>MGSLVCVGTGLQLAGQISVLSRSYIEHADIVFSLLPDGFSQRWLTKLNPNVINLQQFFAQNGEVKNRRDTYEQMVNAILDAVRAGKKTVCALYGHPGVFACVSHMAITRAKAEGFSAKMEPGISAEACLWADLGIDPGNSGHQSFEASQFMFFNHVPDPTTHLLLWQIAIAGEHTLTQFHTSSDRLQILVEQLNQWYPLDHEVVIYEAANLPIQAPRIERLPLANLPQAHLMPISTLLIPPAKKLEYNYAILAKLGIGPEDLG[2x];>[2x]MSGLSDFFTQLGQDAQLMEDYKQNPEAVMRAHGLTDEQINAVMTGDMEKLKTLSGDS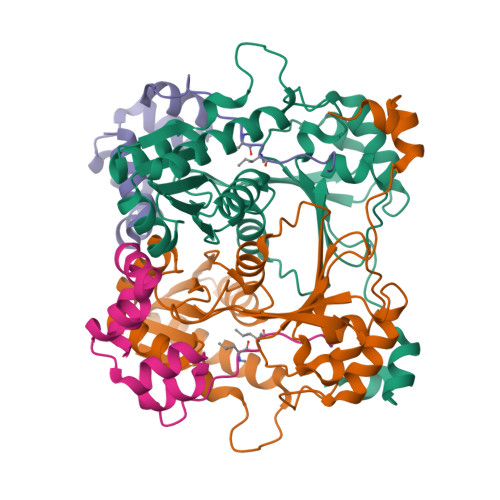SYQSYLVISHGNGD> MMLRTLTRSSAVAG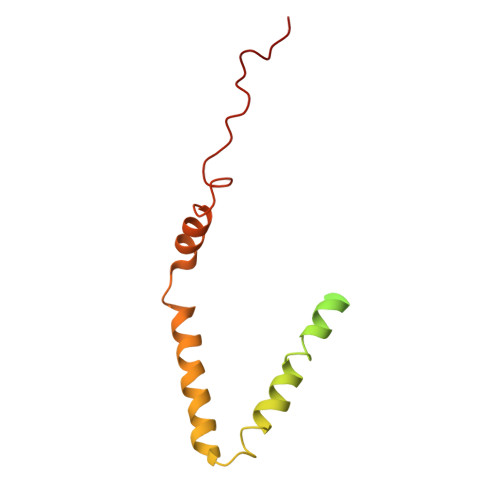QAVRLFKTSAAAAEGNSVAGIIKSVNETSGANLLSSLKTIKAQAAPIYPAAASSTGYSTQAKIALFGALSWILYRADGQSKAHEWIVDLNLNVLQAAWLISFSSLIPFRAVYFAFRGMAPATASTLNGLKTFSSISL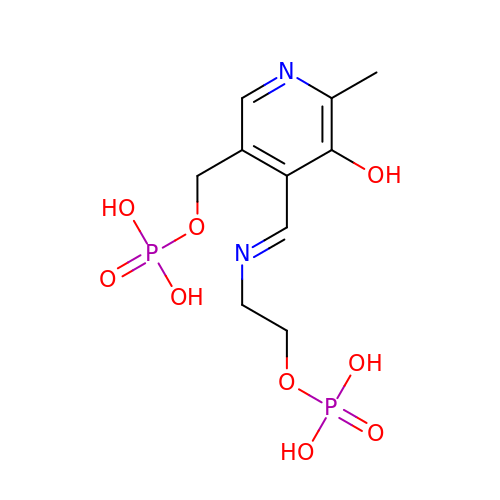{5-hydroxy-6-methyl-4-[(E)-{[2-(phosphonooxy)ethyl]imino}methyl]pyridin-3-yl}methyl dihydrogen phosphate | C10 H16 N2 O9 P2 | AKRAFIXJWODRLT-VZUCSPMQSA-N> MDKKTIYFICTGNSC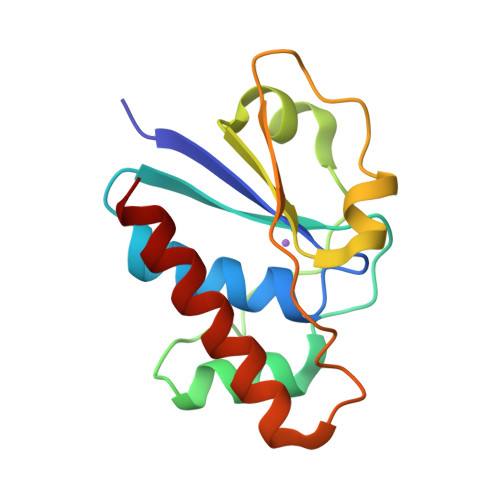RSQMAEGWGKEILGEGWNVYSAGIETHGVNPKAIEAMKEVDIDISNHTSDLIDNDILKQSDLVVTLCSDADNNCPILPPNVKKEHWGFDDPAGKEWSEFQRVRDEIKLAIEKFKLR> NLRNQSYR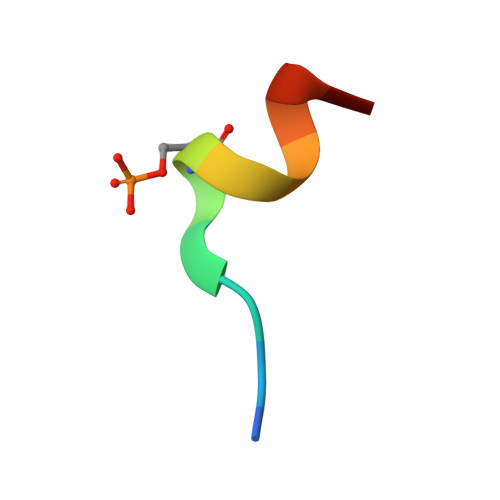AAMK>[4x]KDDLAYSPPFYPSPWADGQGEWAEVYKRAVDIVSQMTLTEKVNLTTGTGWQLERCVGQTGSVPRLNIPSLCLQDSPLGIRFSDYNSAFPAGVNVAATWDKTLAYLRGQAMGEEFSDKGIDVQLGPAAGPLGAHPDGGRNWEGFSPDPAL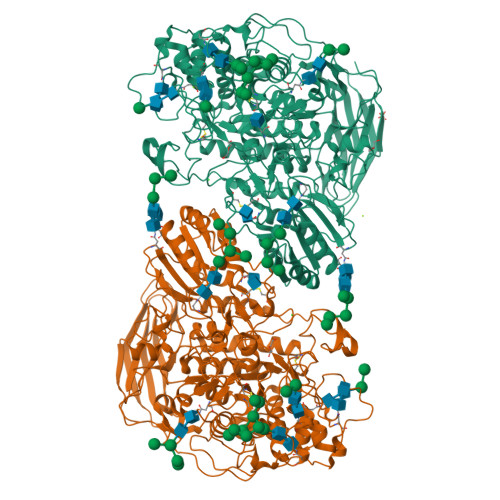TGVLFAETIKGIQDAGVIATAKHYIMNEQEHFRQQPEAAGYGFNVSDSLSSNVDDKTMHELYLWPFADAVRAGVGAVMCSYNQINNSYGCENSETLNKLLKAELGFQGFVMSDWTAHHSGVGAALAGLDMSMPGDVTFDSGTSFWGANLTVGVLNGTIPQWRVDDMAVRIMAAYYKVGRDTKYTPPNFSSWTRDEYGFAHNHVSEGAYERVNEFVDVQRDHADLIRRIGAQSTVLLKNKGALPLSRKEKLVALLGEDAGSNSWGANGCDDRGCDNGTLAMAWGSGTANFPYLVTPEQAIQNEVLQGRGNVFAVTDSWALDKIAAAARQASVSLVFVNSDSGEGYLSVDGNEGDRNNITLWKNGDNVVKTAANNCNNTVVIIHSVGPVLIDEWYDHPNVTGILWAGLPGQESGNSIADVLYGRVNPGAKSPFTWGKTRESYGSPLVKDANNGNGAPQSDFTQGVFIDYRHFDKFNETPIYEFGYGLSYTTFELSDLHVQPLNASRYTPTSGMTEAAKNFGEIGDASEYVYPEGLERIHEFIYPWINSTDLKASSDDSNYGWEDSKYIPEGATDGSAQPRLPASGGAGGNPGLYEDLFRVSVKVKNTGNVAGDEVPQLYVSLGGPNEPKVVLRKFERIHLAPSQEAVWTTTLTRRDLANWDVSAQDWTVTPYPKTIYVGNSSRKLPLQASLPKAQ> ATYQVFPWGTNDPSKGSRTIETDPADKTASEFTWQGNGKTTYTMTEGNNGIAQANYDGDNSWTNDYRPDAPGAKFEYGYSLAETNPKKYIDASVTQLFYTANMYHDMLHALGFNEAAGNFETNNNGAGGKGNDAV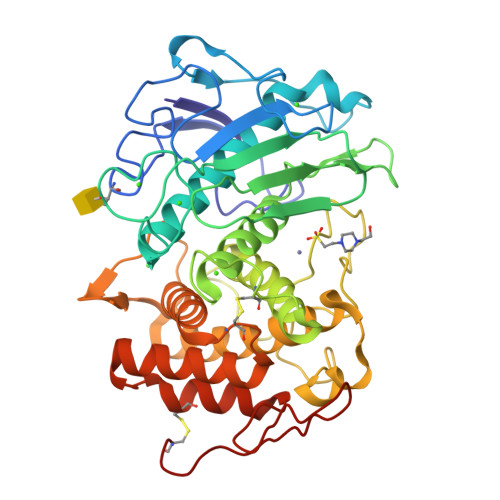ILNAQDGSGTNNANFATPPDGQPGVMRMYIWDESTPYRDCSFDAGVIIHEYTHGVSNRLTGGPANTGCLNVLEAGGMGEGWGDFMAIAIHLKKADTRAKNYPMGDWIANDPKGIRNYLYSTSLTTNPYTYKSVNTMSAVHTIGTVWATILYEVLWNLVEKHGNSEARQPTFNGKVPTDGKFLTMKLVLDGMALQPCSPTFVQARDAIIDADKALTGGSNACELWKAFAKRGLGEGASRGSGSTGRKESTTVPSGVC> SFFDK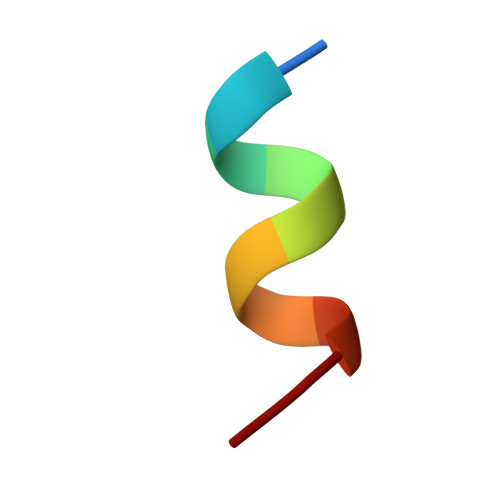KRSER>[2x]MTISLRRTGILKFGIGLVALTIAASVQAKTLVYCSEGSPEGFNPQLFTSGTTYDASSVPIYNRLVEFKIGTTEIEPSLAERWEVSEDGKTYTFYLRKGVKWQDNKDFKPTRDFNADDVIYSFMRQKDDKNPYHKVSGGSYEYFQGMGMGDLITNVVKVDDNTVRFELTRPESPFLADLAMDFASILSAEYADNMLKAGTPEKVDLNPIGTGPFQLQQYQKDSRILYKAFPGFWGTKPKIDRLVFSITPDASVRYAKLQKNECQIMPYPNPADIARMKEDKTINLMEQPGLNVGYLSFNIEKKPLDNLKVRQALTMAVNKDAIIDAVYQGAGQAAKNLIPPTMWGYNDDVKDYAYDPAKAKELLKEAGLPDGFSIDL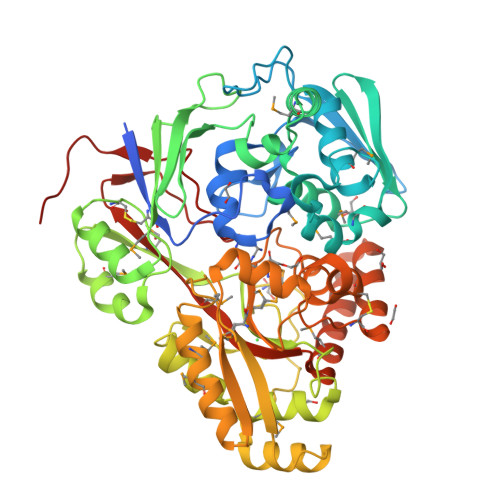WAMPVQRPYNPNARRMAEMIQSDWAKIGVKAKIVTYEWGEYLKRAKDGEHETVMMGWTGDNGDPDNFFATLFSCDAAKQGSNYSKWCYKPFEDLIQPARAEADHDKRVALYKQAQVVMNEQAPALIIAHSTVYEPVRKEVKGYVVDPLGKHHFDNVSLDAGENLYFQ> MGSSHHHHHHSQDPMASVTLSEAEKVYIVHGVQEDLRVDGRGCEDYRCVEVETDVVSNTSGSARVKLGHTDILVGVKAEMGTPKLEKPNEGYLEFFVDCSASATPEFEGRGGDDLGTEIANTLYRIFNNKSSVDLKTLCISPREHCWVLYVDVLLLECGGNLFDAISIAVKAALFNTRIPRVRVLEDEEGSKDIELSDD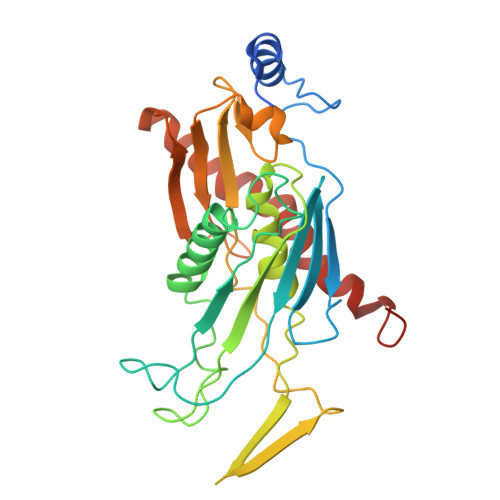PYDCIRLSVENVPCIVTLCKIGYRHVVDATLQEEACSLASLLVSVTSKGVVTCMRKVGKGSLDPESIFEMMETGKRVGKVLHASLQSVVHKEESLGPKRQKVGFLG A key component, the RNA-dependent RNA polymerase [(RdRp), also known as nsp12], catalyzes the synthesis of viral RNA and thus plays a central role in the replication and transcription cycle of COVID-19 virus, possibly with the assistance of nsp7 and nsp8 as cofactors. Therefore, nsp12 is considered a primary target for nucleotide analog antiviral inhibitors such as remdesivir, which shows potential for the treatment of COVID-19 viral infections. The structure of the COVID-19 virus nsp12 contains a right-hand RdRp domain (residues S367 to F920) and a nidovirus-specific N-terminal extension domain (residues D60 to R249) that adopts a nidovirus RdRp-associated nucleotidyltransferase (NiRAN) architecture. The polymerase domain and NiRAN domain are connected by an interface domain (residues A250 to R365).

To inform drug design, we determined the structure of nsp12, in complex with its cofactors nsp7 and nsp8, by cryo–electron microscopy (cryo-EM) using two different protocols: one in the absence of dithiothreitol (DTT) and the other in the presence of DTT. We have also observed C301 to C306 and C487 to C645 form disulfide bonds in the absence of DTT. After the collection and processing of 7994 micrograph movies, we obtained a 2.9-Å resolution three-dimensional reconstruction of an nsp12 monomer in complex with one nsp7-nsp8 pair and an nsp8 monomer, as was previously observed for SARS-CoV. The cryo-EM map allowed us to build the complete structure of COVID-19 virus nsp12, including all residues except S1 to D3 and G897 to D910. In the COVID-19 virus structure, we additionally resolved residues A4 to R118. These constitute a structural block with five antiparallel β strands and two helices. Therefore, we identify residues A4 to T28 and Y69 to R249 as the complete coronaviral NiRAN domain. With the resolution of N-terminal residues, we are also able to identify an N-terminal β hairpin (D29 to K50). The catalytic metal ions, which are observed in several structures of viral polymerases that synthesize RNA, are not observed in this work in the absence of primer-template RNA and nucleoside triphosphates (NTPs).

> SADAQSFLNRVCGVSAARLTPCGTGTSTDVVYRAFDIYNDKVAGFAKFLKTNCCRFQEKDEDDNLIDSYFVVKRHTFSNYQHEETIYNLLKDCPAVAKHDFFKFRIDGDMVPHISRQRLTKYTMADLVYALRHFDEGNCDTLKEILVTYNCCDDDYFNKKDWYDFVENPDILRVYANLGERVRQALLKTVQFCDAMRNAGIVGVLTLDNQDLNGNWYDFGDFIQTTPGSGVPVVDSYYSLLMPILTLTRALTAESHVDTDLTKPYIKWDLLKYDFTEERLKLFDRYFKYWDQTYHPNCVNCLDDRCILHCANFNVLFSTVFPPTSFGPLVRKIFVDGVPFVVSTGYHFRELGVVHNQDVNLHSSRLSFKELLVYAADPAMHAASGNLLLDKRTTCFSVAALTNNVAFQTVKPGNFNKDFYDFAVSKGFFKEGSSVELKHFFFAQDGNAAISDYDYYRYNLPTMCDIRQLLFVVEVVDKYFDCYDGGCINANQVIVNNLDKSAGFPFNKWGKARLYYDSMSYEDQDALFAYTKRNVIPTITQMNLKYAISAKNRARTVAGVSICSTMTNRQFHQKLLKSIAATRGATVVIGTSKFYGGWHNMLKTVYSDVENPHLMGWDYPKCDRAMPNMLRIMASLVLARKHTTCCSLSHRFYRLANECAQVLSEMVMCGGSLYVKPGGTSSGDATTAYANSVFNICQAVTANVNALLSTDGNKIADKYVRNLQHRLYECLYRNRDVDTDFVNEFYAYLRKHFSMMILSDDAVVCFNSTYASQGLVASIKNFKSVLYYQNNVFMSEAKCWTETDLTKGPHEFCSQHTMLVKQGDDYVYLPYPDPSRILGAGCFVDDIVKTDGTLMIERFVSLAIDAYPLTKHPNQEYADVFHLYLQYIRKLHDELTGHMLDMYSVMLTNDNTSRYWEPEFYEAMYTPHTVLQHHHHHHHHHH;>AIASEFSSLPSYAAFATAQEAYEQAVANGDSEVVLKKLKKSLNVAKSEFDRDAAMQRKLEKMADQAMTQMYKQARSEDKRAKVTSAMQTMLFTMLRKLDNDALNNIINNARDGCVPLNIIPLTTAAKLMVVIPDYNTYKNTCDGTTFTYASALWEIQQVVDADSKIVQLSEISMDNSPNLAWPLIVTALRANSAVKLQ[2x];> SKMSDVKCTSVVLLSVLQQLRVESSSKLWAQCVQLHNDILLAKDTTEAFEKMVSLLSVLLSMQGAVDINKLCEEMLDNRATLQ> MRLLTALFAYFIVALILAFSVSAKSMSERRAVYIGALFPMSGGWPGGQACQPAVEMALEDVNSRRDILPDYELKLIHHDSKCDPGQATKYLYELLYNDPIKIILMPGCSSVSTLVAEAARMWNLIVLSYGSSSPALSNRQRFPTFFRTHPSATLHNPTRVKLFEKWGWKKIATIQQTTEVFTSTLDDLEERVKEAGIEITFRQSFFSDPAVPVKNLKRQDARIIVGLFYETEARKVFCEVYKERLFGKKYVWFLIGWYADNWFKIYDPSINCTVDEMTEAVEGHITTEIVMLNPANTRSISNMTSQEFVEKLTKRLKRHPEETGGFQEAPLAYDAIWALALALNKTSGGGGRSGVRLEDFNYNNQTITDQIYRAMNSSSFEGVSGHVVFDASGSRMAWTLIEQLQGGSYKKIGYYDSTKDDLSWSKTDKWIGGSPPADQTLVIKTFRFLSQKLFISVSVLSSLGIVLAVVCLSFNIYNSHVRYIQNSQPNLNNLTAVGCSLALAAVFPLGLDGYHIGRNQFPFVCQARLWLLGLGFSLGYGSMFTKIWWVHTVFTKKEEKKEWRKTLEPWKLYATVGLLVGMDVLTLAIWQIVDPLHRTIETFAKEEPKEDIDVSILPQLEHCSSRKMNTWLGIFYGYKGLLLLLGIFLAYETKSVSTEKINDHRAVGMAIYNVAVLCLITAPVTMILSSQQDAAFAFASLAIVFSSYITLVVLFVPKMRRLITRGEWQSEAQDTMKTGSSTNNNEEEKSRLLEKENRELEKSGRLEVLFQ;> MASPRSSGQPGPPPPPPPPPARLLLLLLLPLLLPLAPGAWGWARGAPRPPPSSPPLSIMGLMPLTKEVAKGSIGRGVLPAVELAIEQIRNESLLRPYFLDLRLYDTECDNAKGLKAFYDAIKYGPNHLMVFGGVCPSVTSIIAESLQGWNLVQLSFAATTPVLADKKKYPYFFRTVPSDNAVNPAILKLLKHYQWKRVGTLTQDVQRFSEVRNDLTGVLYGEDIEISDTESFSNDPCTSVKKLKGNDVRIILGQFDQNMAAKVFCCAYEENMYGSKYQWIIPGWYEPSWWEQVHTEANSSRCLRKNLLAAMEGYIGVDFEPLSSKQIKTISGKTPQQYEREYNNKRSGVGPSKFHGYAYDGIWVIAKTLQRAMETLHASSRHQRIQDFNYTDHTLGRIILNAMNETNFFGVTGQVVFRNGERMGTIKFTQFQDSREVKVGEYNAVADTLEIINDTIRFQGSEPPKDKTIILEQLRKISLPLYS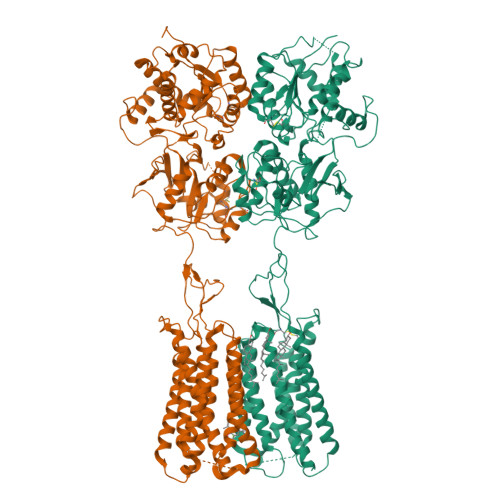ILSALTILGMIMASAFLFFNIKNRNQKLIKMSSPYMNNLIILGGMLSYASIFLFGLDGSFVSEKTFETLCTVRTWILTVGYTTAFGAMFAKTWRVHAIFKNVKMKKKIIKDQKLLVIVGGMLLIDLCILICWQAVDPLRRTVEKYSMEPDPAGRDISIRPLLEHCENTHMTIWLGIVYAYKGLLMLFGCFLAWETRNVSIPALNDSKYIGMSVYNVGIMCIIGAAVSFLTRDQPNVQFCIVALVIIFCSTITLCLVFVPKLITLRTNPDAATQNRRFQFTQNQKKEDSKTSTSVTSVNQASTSRSGRGGSENLYFQGGSGSGGDYKDDDDKDYKDDDDK> SMGKLSEQLKHCNGI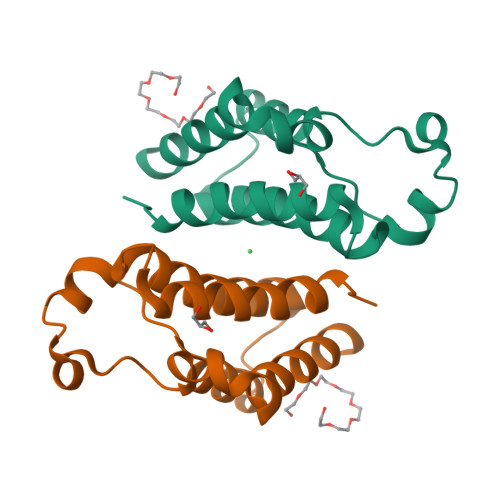LKELLSKKHAAYAFPFYKPVDASALGLHDYHDIIKHPMDLSTVKRKMENRDYRDAQEFAADVRLMFSNCYKYNPPDHDVVAMARKLQDVFEFRYAKMPD> GSSATSGLQAYVDSYDGYEFLYPRGWVQVQVEDPVDVVFHDIIETTEN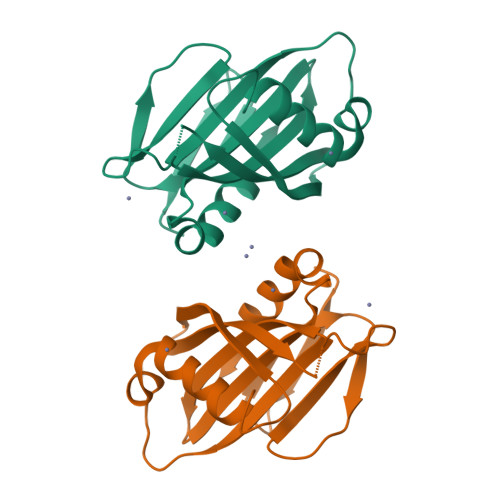VSVVVNTVASTKSLEELGSPEEVGDRLLRNIIAPSESGRSSALIAATSQKADDKTYYILEYAVTLPGDGNTAQQRHNLSSIAVSRGKVYTLSVSAPEERWPKVEDQFKTIVSSFTVY>[2x]HHHHHHMRVSFMVAM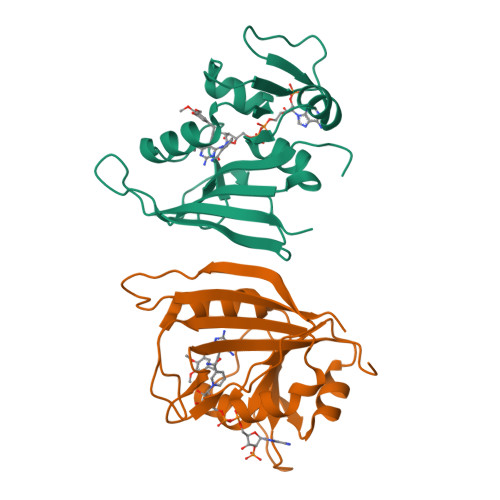DENRVIGKDNNLPWRLPSELQYVKKTTMGHPLIMGRKNYEAIGRPLPGRRNIIVTRNEGYHVEGCEVAHSVEEVFELCKNEEEIFIFGGAQIYDLFLPYVDKLYITKIHHAFEGDTFFPEMDMTNWKEVFVEKGLTDEKNPYTYYYHVYEKQQ>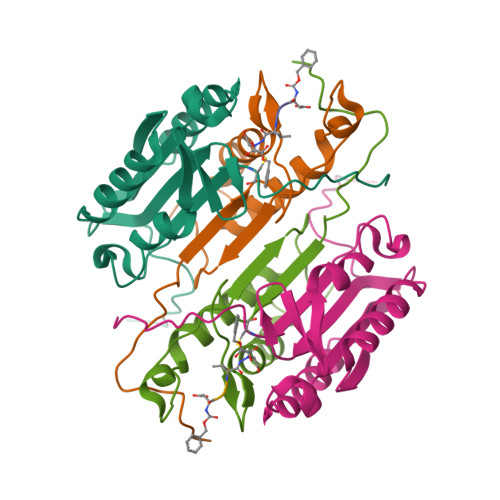 SGISLDNSYKMDYPEMGLCIIINNKNFHKSTGMTSRSGTDVDAANLRETFRNLKYEVRNKNDLTREEIVELMRDVSKEDHSKRSSFVCVLLSHGEEGIIFGTNGPVDLKKITNFFRGDRCRSLTGKPKLFIIQACRGTELDCGIETD;> ASGVDDDMACHKIPVEADFLYAYSTAPGYYSWRNSKDGSWFIQSLCAMLKQYADKLEFMHILTRVNRKVATEFESFSFDATFHAKKQIPCIVSMLTKELYFYH1,1'-binaphthalene-2,2'-dicarboxylic 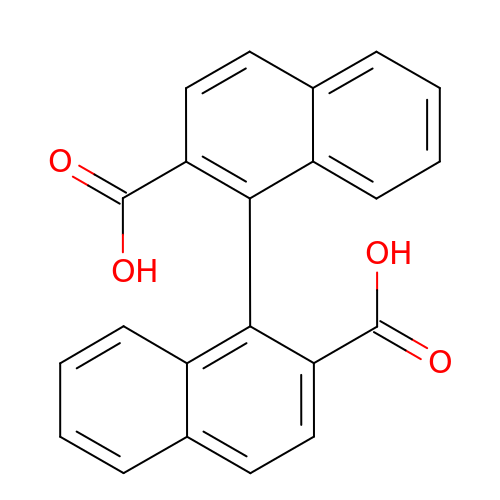acid | C22 H14 O4 | YDZNRNHKJQTGCG-UHFFFAOYSA-N> MGSDKIHHHHHHMKIHFVGIGGIGMSAVALHEFSNGNDVYGSNIEETERTAYLRKLGIPIFVPHSADNWYDPDLVIKTPAVRDDNPEIVRARMERVPIENRLHYFRDTLKREKKEEFAVTGTDGKTTTTAMVAHVLKHLRKSPTVFLGGIMDSLEHGNYEKGNGPVVYELDESEEFFSEFSPNYLIITNARGDHLENYG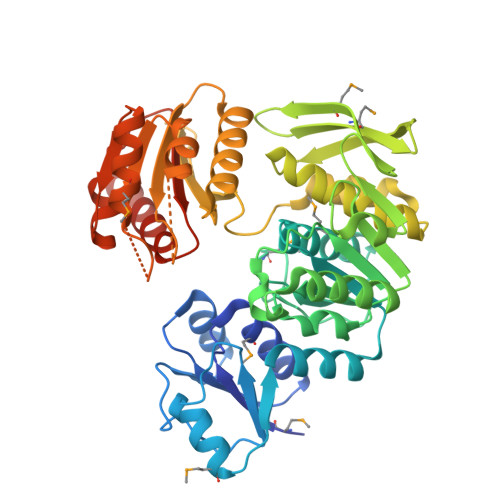NSLTRYRSAFEKISRNTDLVVTFAEDELTSHLGDVTFGVKKGTYTLEMRSASRAEQKAMVEKNGKRYLELKLKVPGFHNVLNALAVIALFDSLGYDLAPVLEALEEFRGVHRRFSIAFHDPETNIYVIDDYAHTPDEIRNLLQTAKEVFENEKIVVIFQPHRYSRLEREDGNFAKALQLADEVVVTEVYDAFEEKKNGISGKMIWDSLKSLGKEAYFVEKLPELEKVISVSENTVFLFVGAGDIIYSSRRFVERYQSSKSSPSRVLGSNK>AHHHHHHMRIGHGYDVHRFGEGDFITLGGVRIPHKHGLVAHSDGDVLLHALSDALLGAAALGDIGKHFPDTDPRFKGADSRALLRHVVAIVAEKGWKVGNVDATIVAQAPKMAPHIETMRGLIAEDLGVAVDQVNVKATTTE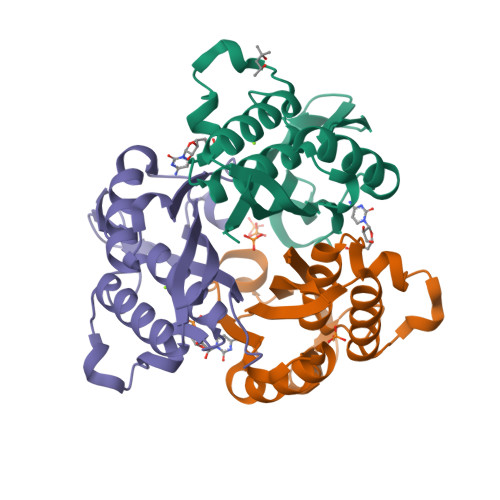RLGFTGREEGIAVHAVALLMAR[3x]>MRGSHHHHHHGSMMSEIIAVANQKGGVGKTTTAVNLAASLAVHEKKILLIDFDPQANATSSLGFRRDKIDYDIYHVLIGRKQISQVILKTQMPFLDLVPSNLGLAGFEKTFYDSQDENKRGELMLKNALESVVGLYDYIIIDSPPALGPLTINSLSAA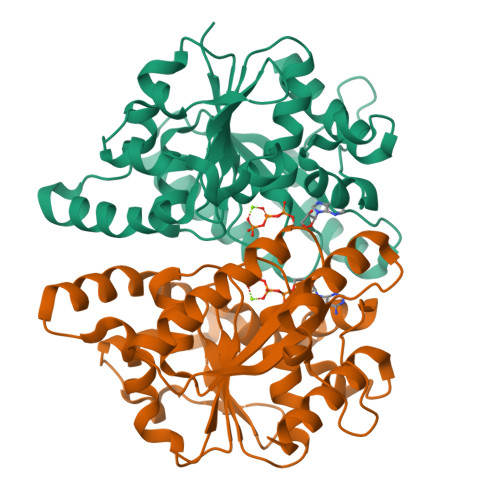HSVIIPIQCEFFALEGTKLLLNTIRMLQKSTNPKLKIRGFLPTMHVPQLNLTKGVLAELFKYFDSEFFRDSATGEYIMIPKSVKLAESPSFGKPILLYDIKSNGSIAYQKLAQSILQG[2x]6-oxidanylidene-6-phenyl-hexanoic acid | C12 H14 O3 | 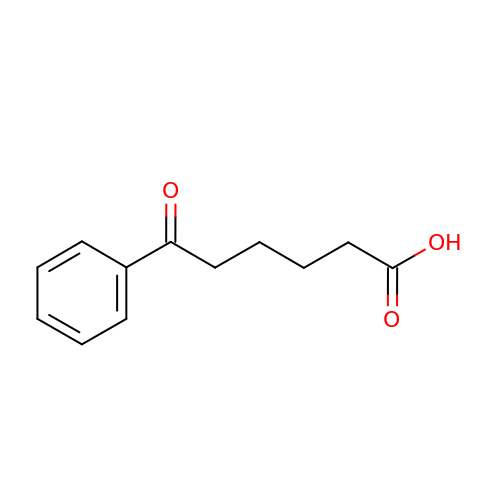AIEMSTCGCMIJTI-UHFFFAOYSA-N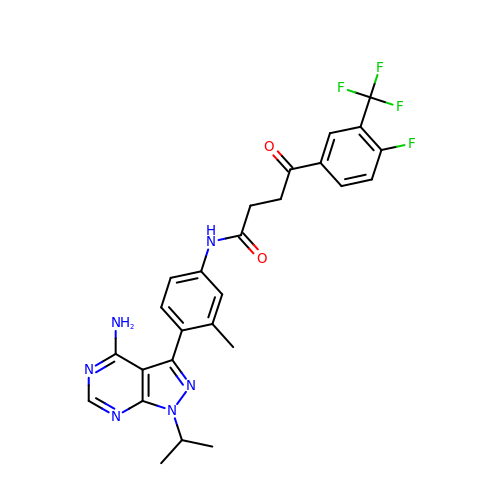~{N}-[4-(4-azanyl-1-propan-2-yl-pyrazolo[3,4-d]pyrimidin-3-yl)-3-methyl-phenyl]-4-[4-fluoranyl-3-(trifluoromethyl)phenyl]-4-oxidanylidene-butanamide | C26 H24 F4 N6 O2 | QTIJDEKGLBXUPB-UHFFFAOYSA-N(4R)-6-[3-(benzyloxy)phenyl]-4-methyl-1,3,4,5-tetrahydro-2H-1,5-benzodiazepin-2-one 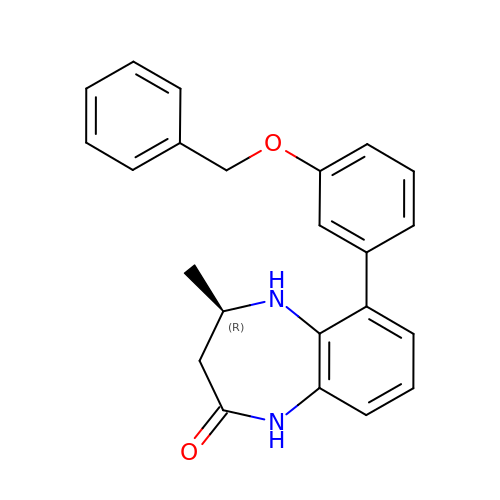| C23 H22 N2 O2 | XKIQUMIGIBMUJB-MRXNPFEDSA-N> SREFDFFTYETPKVIVVKSWTIGIINRVVQLLIISYFVGWVFLHEKAYQVRDTAIESSVVTKVKGSGLYANRVMDVSDYVTPPQGTSVFVIITKMIVTENQMQGFCPESEEKYRCVSDSQCGPERLPGGGILTGRCVNYSSVLRTCEIQGWCPTEVDTVETPIMMEAENFTIFIKNSIRFPLFNFEKGNLLPNLTARDMKTCRFHPDKDPFCPILRVGDVVKFAGQDFAKLARTGGVLGIKIGWVCDLDKAWDQCIPKYSFTRLDSVSEKSSVSPGYNF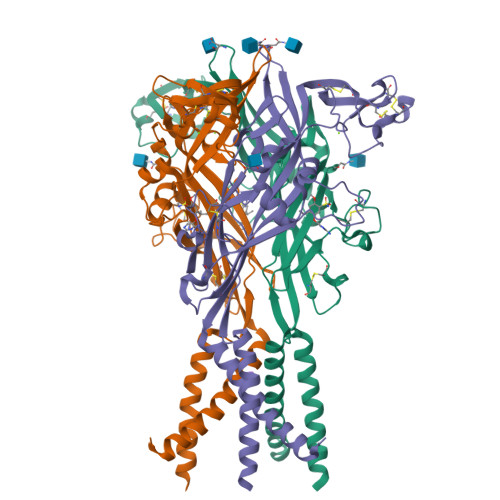RFAKYYKMENGSEYRTLLKAFGIRFDVLVYGNAGKFNIIPTIISSVAAFTSVGVGTVLCDIILLNFLKGADQYKAKKFEEVNET>[2x]MGGSHHHHHHSRAWRHPQGGSHHHHHHGMRDLYDDDDKDPPEISPHAPASADATRIAAIVAARQDIPGALLPILHEIQDTQGYIPDAAVPVIARALNLSRAEVHGVITFYHHFRQQPAGRHVVQVCRAEACQSVGAEALAEHAQRALGCGFHETTADGQVTLEPVYCLGQCACGPAVMVGEQLHGYVDARRFDALVRSLRESSAEKTTEAAEAQA;>[2x]MITITTIFVPRDSTA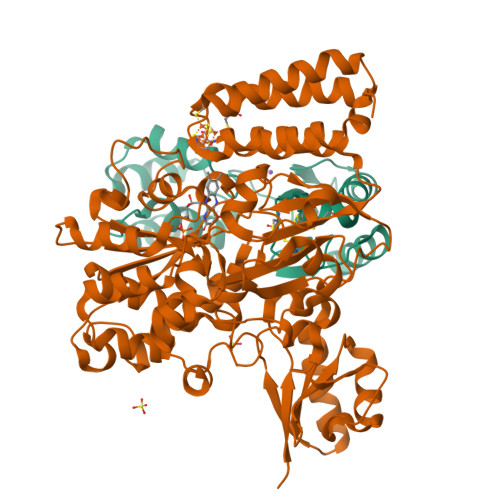LALGADDVARAIAREAAARNEHVRIVRNGSRGMFWLEPLVEVQTGAGRVAYGPVSAADVPGLFDAGLLQGGEHALSQGVTEEIPFLKQQERLTFARVGITDPLSLDDYRAHEGFAGLERALAMQPAEIVQEVTDSGLRGRGGAAFPTGIKWKTVLGAQSAVKYIVCNADEGDSGTFSDRMVMEDDPFMLIEGMTIAALAVGAEQGYIYCRSEYPHAIAVLESAIGIANAAGWLGDDIRGSGKRFHLEVRKGAGAYVCGEETALLESLEGRRGVVRAKPPLPALQGLFGKPTVINNVISLATVPVILARGAQYYRDYGMGRSRGTLPFQLAGNIKQGGLVEKAFGVTLRELLVDYGGGTRSGRAIRAVQVGGPLGAYLPESRFDVPLDYEAYAAFGGVVGHGGIVVFDETVDMAKQARYAMEFCAIESCGKCTPCRIGSTRGVEVMDRIIAGEQPVKHVALVRDLCDTMLNGSLCAMGGMTPYPVLSALNEFPEDFGLASNPAKAA>[12x]GFFSFIGEAFQGAGDMWRAYTDMKEAGWKDGDKYFHARGNYDAAQRGPGGVW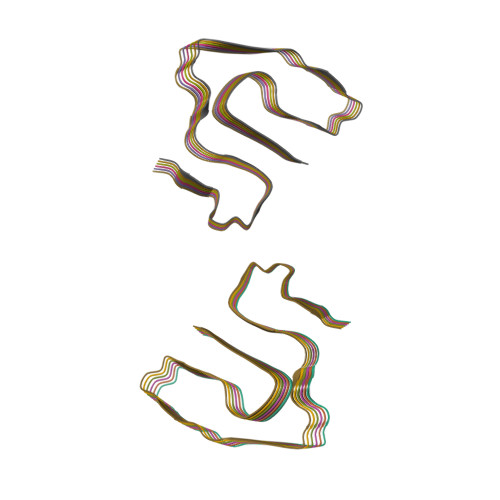AAEKISDARESFQEFFGRGHEDTMADQEANRHGRSGKDPNYYRPPGLPAKY>VPEAPTPMWPDDLQNHTFLHTVYCQDGSPSVGLSEAYDEDQLFFFDFSQNTRVPRLPEFADWAQEQGDAPAILFDKEFCEWMIQQIGPKLDGKIPVSRGFPIAEVFTLKPLEFGKPNTLVCFVSNLFPPMLTVNWQHHSVPVEGFGPTFVSAVDGLSFQAFSYLNFTPEPSDIFSCIVTHEIDRYTAIAYWVPRNALPSDLLEDYKDDDDK[2x];>[2x]GGFVAHVESTCLLDDAGTPKDFTYCISFNKDLLTCWDPEENKMAPCEFGVLNSLANVLSQHLNQKDTLMQRLRNGLQNCATHTQPFWGSLTNRTRPPSVQVAKTTPFNTREPVMLACYVWGFYPAEVTITWRKNGKLVMPHSSAHKTAQPNGDWTYQTL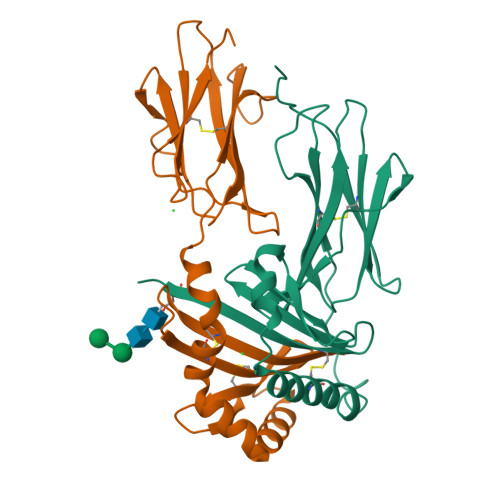SHLALTPSYGDTYTCVVEHIGAPEPILRDWTPGLSPMQTLKKPPTPPPEPET> GSGSAKYTYRSLGRHLDFLRPGLRFGGSQSSKYTYYTVEVKIDTVNLPLYKDSRSLDPHVTGTFTIKNLTPVLDKVVTLFEGYVINYNQFPLCSLHWPAEETLD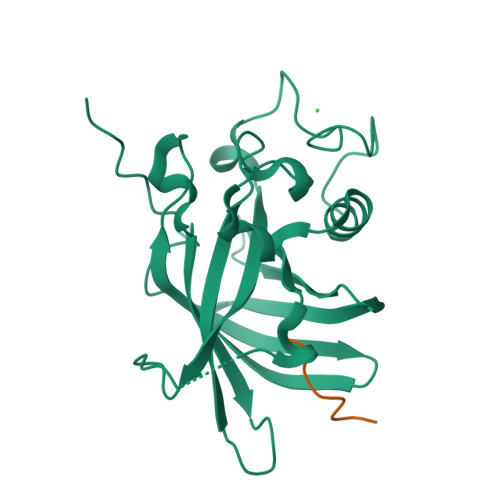PYMAQRESDCSHWKRFGHFGSDNWSLTERNFGQYNHESAEFMNQRYIYLKWKERFLLDDEEQENLMLDDNHHLEGASFEGFYYVCLDQLTGSVEGYYYHPACELFQKLELVPTNCDALNT;> FWLPANLW>[2x]MAFNPAPKAVQENHHVDYVIRFNYGDIDTPEAIKKFEVLLLELSEVGLQTEVRQGDENSLFVFVRAASKKKLKRAVYQSRVRDWLYGVRNTEPEPASSAKPQSEAERLLVIYHLITVPKAEGGAGITPRHGEWKNVDAIFPLHDEETNRQCMREWSKKTFLSTEDLDRIRNTFGEHVGFYFAFLQSYFRFLMFPAAFGFSCWLLLGSFSIIYTVVNCLWCIVFIEYWKRQEEDLSCRWQTKGVSAVHEKRAEFKPEKEIRDESTGEVRGVFPATKRMYRQLLQVPFALLAAVALGAIIATCFAIEIFISEVYNGPLKGYLVFIPTILVSALIPTMSAVLLTVATKLNDYENYETQDAYKVALTQKIFVVNFITSYLPIILTAFVYVPFASRIVPYLDVFHLTVRPFVSKEHAIKARTEFSINPDRLRKQVIYFTVTAQIVGFALETIVPFVKQRVFREYKEYTKKQHAKAEPGNGAGEKKTVSLGDDEDEARFLTRVRNEAELEDYDVTDDLREMCIQFGYLALFSPVWPLVPVSFLINNWVELRSDFFKICVECKRPWPQRADTIGPWLDSLGFLSWVGSITSSALVYMFSNGHEGPNGEPTTIRCWALLLTIFFSEHLYLIVRYAVRSALAKLEPPNTRRERIERFMMRKRYLDTVLSAESDDDADEVKGVVSSIPPSEITRESLEQDARDWSKQGTDPTERFWMRQRGWKESAEVGLSLITKAKGDETKKQQ

TMEM16 scramblases dissipate the plasma membrane lipid asymmetry to activate multiple eukaryotic cellular pathways. The TMEM16 superfamily is comprised of Cl- channels and dual function scramblases/non-selective ion channels. Our results show afTMEM16 thins the membrane to enable scrambling and that an open hydrophilic pathway is not a structural requirement to allow rapid transbilayer movement of lipids. Scrambling by the TMEM16’s is modulated by two signals, binding of Ca2+ facilitates opening of the groove while the properties of the membrane determine whether the scramblase can thin the membrane enough to enable lipid flipping.

The 3.5 Å resolution structure of afTMEM16 in the larger MSP2N2 nanodiscs in C22/Ca2+ shows an open permeation pathway in all 3D reconstructions, with Cα r.m.s.d. ~0.5 Å to C18/Ca2+ and ~0.4 Å to C22/Ca2+MSP1E3. Thus, in afTMEM16 an open groove is not sufficient to enable lipid scrambling and nanodisc size does not influence the conformation. In the C22/Ca2+ maps we resolved several lipids near the dimer interface corresponding to D2, D3, D6, and D7 (in MSP1E3 map) and to D2 and D6 (in MSP2N2 map) seen in the C18/Ca2+ map. Reconstituting afTMEM16 in membranes formed from lipids with longer acyl chains dramatically inhibits scrambling although the groove remains open.> AHLESLTHPGSKVTFPIDQDISATPQNPNLKVFFFAIDNCLYKSSTRIHDLMQQSILRFFQTHLKLSPEDAHVLNNSYYKEYGLAIRGLVMFHKVNALEYNRLVDDSLPLQDILKPDIPLRNMLLRLRQSGKIDKLWLFTNAYKNHAIRCLRLLGIADLFDGLTYCDYSRTDTLVCKPHVKAFEKAMKESGLARYENAYFIDDSGKNIETGIKLGMKTCI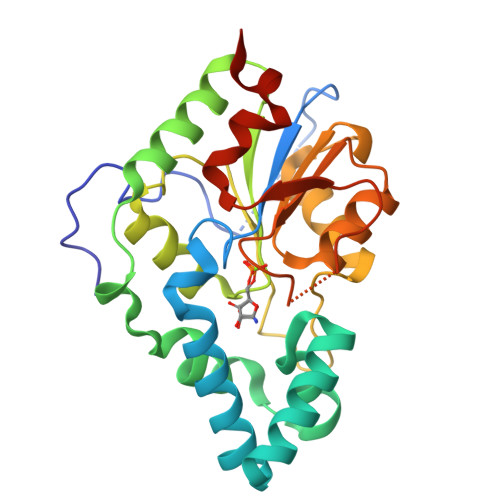HLVENEVNEILGQTPEGAIVISDILELPHVVSDLFLEHHHHHH>NNLQNIIYNPVIPFVGTIPDQLDPGTLIVIRGHVPSDADRFQVDLQNGSSMKPRADVAFHFNPRFKRAGCIVCNTLINEKWGREEITYDTPFKREKSFEIVIMVLKDKFQVAVNGKHTLLYGHRIGPEKIDTLGIYGKVNIHSIGFSFSSD[2x]

pmcGalectins are a family of proteins that bind β-d-galactopyranoside-containing glycoconjugates through their canonical carbohydrate recognition domains (CRDs). Galectin-8 is a divalent galectin found in the liver, the kidney, the cardiac muscle, the lung, and the brain. Galectin-8 is a carbohydrate-binding protein that plays a crucial role in tumor progression and metastasis, antibacterial autophagy, modulation of the immune system, and bone remodeling. However, there are major differences between the two CRDs, such as the presence of Arg45, Arg59, Tyr141, and Gln47 in the N-terminal CRD (galectin-8N) and the presence of Ser255, Asn257, and Asn348 in the C-terminal CRD (galectin-8C).

Galectin-8N was first cocrystallized with lactose, and then the ligands were soaked into galectin-8N-lactose crystals, followed by collection of X-ray diffraction data at 1.52 and 2.1 Å resolution for the galectin-8N–6a complex and galectin-8N–9 complex, respectively. Both complexes showed that the O4 and O6 of the d-galactal portion bind to galectin-8N in a similar manner as the corresponding oxygens in the d-galactosides. Namely, the O4 of the d-galactal is involved in a hydrogen-bonding network with Arg45, Arg69, and His65. Further, the O6 of the d-galactal engages in hydrogen bonding interactions with Asn79 and Glu89, while the O3 engages in a hydrogen bonding interaction with Arg45. As for the galectin-8N–6a complex, the five-membered ring of the benzimidazole ring is placed in a favorable position to engage in cation−π stacking with Arg45 while the basic nitrogen of the benzimidazole engages in a dipole–dipole interaction with Gln 47 and Arg59. The carboxylate moiety of the benzimidazole establishes a water-mediated hydrogen bond with Gly142. The endocyclic double bond of the d-galactal moiety in both complexes is placed in proximity to the guanidinium side chains of Arg45 and Arg69. A NH LUMO of Arg45 overlapped with the HOMOs of O4 and the d-galactal double bond. Hence, a favorable interaction between one of the Arg45 protons and the d-galactal double bond likely contributes to improved affinity of galectin-8N for d-galactal derivatives. Compound 6a is the most selective galectin-8N ligand to date with 15-fold selectivity over galectin-3.Carbohydrate-binding modules (CBMs) are non-catalytic proteins found appended to carbohydrate-active enzymes. Soil and marine bacteria secrete such enzymes to scavenge nutrition, and they often use CBMs to improve reaction rates and retention of released sugars. Here we present a structural and functional analysis of the recently established CBM family 92. All proteins analysed bind preferentially to β−1,6-glucans.

To probe the mode of binding of CBM92 domains, we successfully determined the protein structures of the C. pinensis proteins CpCBM92A and CpCBM92B by macromolecular crystallography. As was predicted by sequence analysis, both proteins form a β-trefoil structure comprised of 12 β-strands arranged into 3 subdomains (α, β, and γ), similar to β-trefoil domains found in Fascin and CBM13 proteins. The binding cleft Arg residue in the β-subdomain of CpCBM92B is found in subdomains β and γ in both CpCBM92A and -B, but is substituted with a Ser in the binding clefts of subdomain α in both proteins. This substitution in the α site leads to a substantial increase in accessibility around the glucosyl unit’s O2, which may permit binding to oligo- or polysaccharide extensions from this position. We also see that the α site knockout shows only a small loss of binding ability compared to the wild type, but that there is some residual binding in the β/γ site variant W523A/W565A, suggesting that the wild type α site does make some small contribution to binding in the full protein. The α binding site of CpCBM92A differs from the other two in that it lacks an otherwise well-conserved adjacent Arg that likely supports binding by interacting with a glucose ligand and by creating a topographic ‘wall’ for the binding site. To probe the respective functions of the three putative glycan binding sites, a series of modified constructs were generated for CpCBM92A, systematically altering the Trp in each WExF motif. Variants with single (W481A α site, W523A β site, W565A γ site variants), double (W481A/W565A, W481/W523A, W523A/W565A), and triple (W481A/W523A/W565A) binding site substitutions were produced using site-directed mutagenesis (red stars in Fig. 3 show the positions of the residues modified). Pull-down assays revealed that the single mutation variants showed the same binding specificities as the wild-type, while the double and triple variants showed impaired or abolished binding, confirming that there are no further unrecognised binding sites in the protein. The loss of the Trp residue from either the β or γ binding site (W523A and W565A variants, respectively) caused a major shift in apparent binding ability, with the loss of the β site having the most profound effect. This indicates that for CpCBM92A, the β site likely has the strongest affinity for the ligand.

> MASMTGGQQMGRGSVGKTIWLQGFNNKYVNSKNGQGAMWCDSDAPQAWELFTVVDAGNGKIALRGNNGMYVSSENGEQAITCNRPAIQGWEAFDWLETADGKVSLRGSNGLFISSENGAAAMTCTRPTASGWEAFGYSVVGNALEHHHHHH> LDI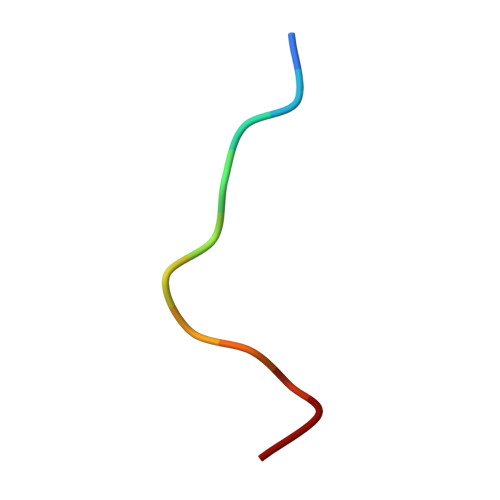PAFLRKQA>GELVRTDSPNFLCSVLPTHWRCNKTLPIAFKVVAKGDVPDGTLVTVMAGNDENYSAELRNATAAMKNQVARFNDLRFVGRSG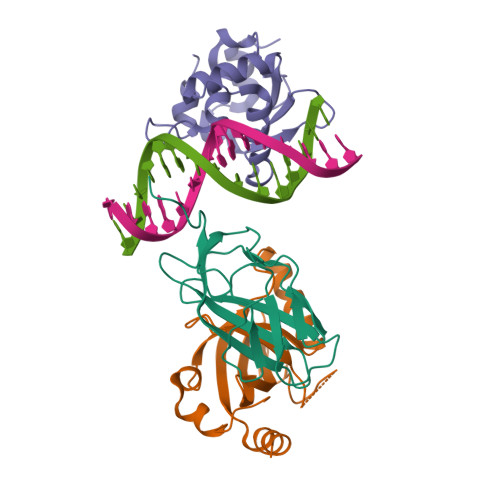RGKSFTLTITVFTNPPQVATYHRAIKITVDGPREPRRHRQKLDDQTKPGSLSFSERLSELEQLRRTAMRVSPHHPAPTPNPRASLNHSTAFNPQPQSQMQDARQIQPSPPWSYDQSYQYLGS[2x];>MPRVVPDQRSKFENEEFFRKLSRECEIKYTGFRDRPHEERQTRFQNACRDGRSEIAFVATGTNLSLQFFPASWQGEQRQTPSREYVDLEREAGKVYLKAPMILNGVCVIWKGWIDLHRLDGMGCLEFDEERAQQEDALAQQA[2x];>SLQRVPSYDSFDSEDYPAALPNHKPKGTFKDYVRDRADLNKDKPVIPAAALAGYTGSPPIQLWQFLLELLTDKSCQSFISWTGDGWEFKLSDPDEVARRWGKRKNKPKMNYEKLSRGLRYYYDKNIIHKTAGKRYVYRFVCDLQSLLGYTPEELHAMLDVKPDADE[2x]> MAYGKAHLEAQLKRALAEEIQALEDPRLFLLTVEAVRLSKDGSVLSVYVEAFREEEGAL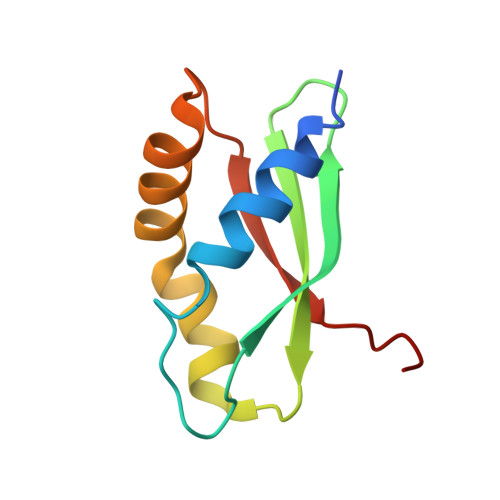RALSRAERRLVAALARRVRMRRLPRLEFLPWRASPA>[4x]EFMNAPLRGQVYRCDLGYGAKPWLIVSNNARNRHTADVVAVRLTTTRRTIPTWVA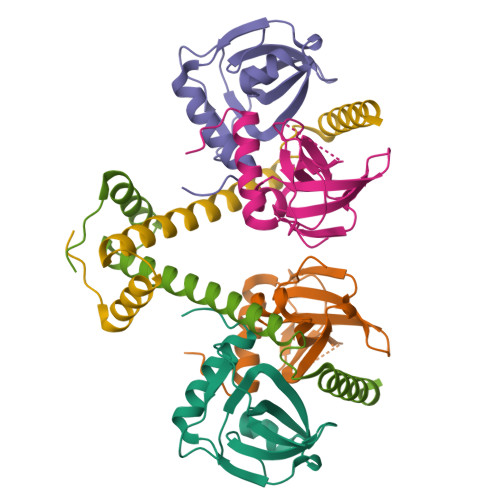MGPSDPLTGYVNADNIETLGKDELGDYLGEVTPATMNKINTALATALGLPWP;>[2x]MTVRLDQQTRQRLQDIVKGGYRSANAAIVDAINKRWEALHDEQLDAAYAAAIHDNPAYPYESEAERSAARARRNARQQRSA>GGYAVDYNEPIIIK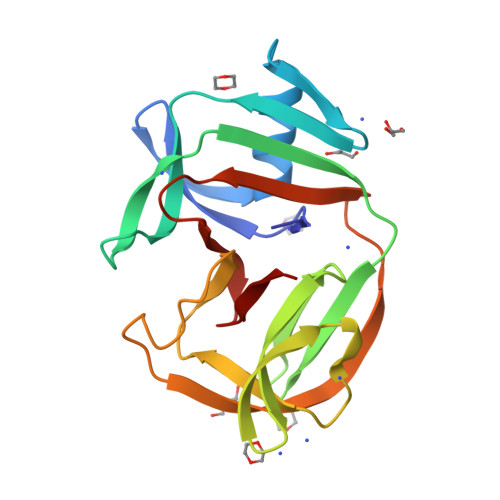ENGEIKVVKIGELIDKIIENSENIRREGILEIAKCKGIEVIAFNSNYKFKFMPVSEVSRHPVSEMFEIVVEGNKKVRVTRSHSVFTIRDNEVVPIRVDELKVGDILVLAKRITNIYTNRKLEKLINSDFIFLKIKEINKVEPTSGYAYDLTVPNAENFVAGFGGFVLHNA[2x]>MTERTLVLIKPDGIERQLIGEIISRIERKGLTIAALQLRTVSAELASQHYAEHEGKPFFGSLLEFITSGPVVAAIVEGTRAIAAVRQLAGGTDPVQAAAPGTIRGDFALETQF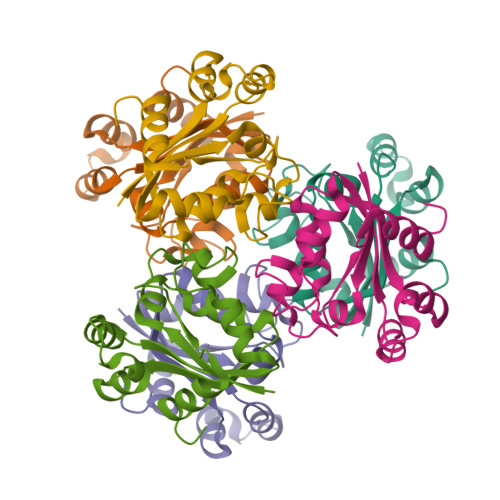NLVHGSDSAESAQREIALWFPGA[6x]> QFRAIIESPEGAGHVGYQYRRNTGSTMRMVSDVLDERVSLWDFHCDPSGNVIQPGPNVDSRQYLQAAIDYVSSNGGGTITIPAGYTWYLGSYGVGGIAGHSGIIQLRSNVNLNIEGRIHLSPFFDLKPFQVFVGFDNGDPASSGNLENCHIYGHGVVDFGGYEFGASSQLRNGVAFGRSYNCSVTGITFQNGDVTWAITLGWNGYGSNCYVRKCRFINLVNSSVNAAHSTVYVNCPYSGVESCYFSMSSSFARNIACSVQLHQHDTFYRGSTVNGYCRGAYVVMHAAEAAGAGSYAYNMQVENNIAVIYGQFVILGSDVTATVSGHLNDVIVSGNIVSI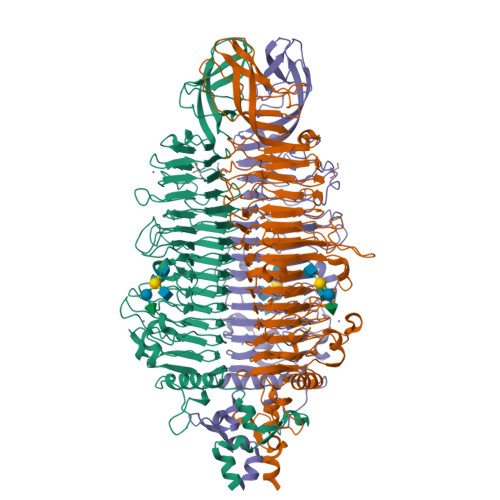GERAAFSAPFGAFIDIGPDNSGASNVQDIQRVLVTGNSFYAPANITDSAAITLRANLNGCTFIANNFDCRYMVYNAPGTTSPVVQNLVWDKSNVIGGTHANQRAGQNLFDMQFASVVNSTIEVQLSCEDLSMFSCILFPASCQLSYSKITVDSAWTKSMSNTAVFEGNQQAGANVYVSYPATVNLTSYNTQGAVPFFSTDTNYAWVTSAYSLSINENLDFSPPATYTNKANGQLVGVGYNEIGGVRSVSVRLMLQRQV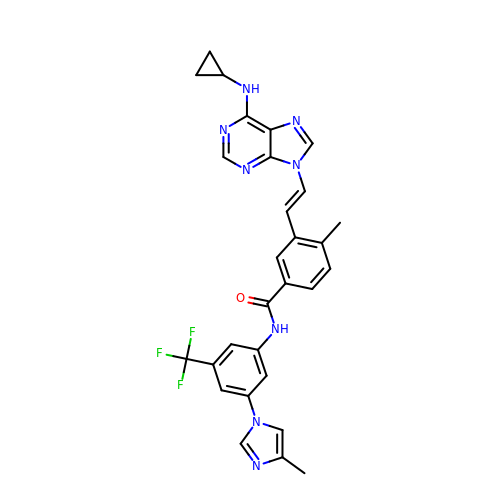3-{(E)-2-[6-(cyclopropylamino)-9H-purin-9-yl]ethenyl}-4-methyl-N-[3-(4-methyl-1H-imidazol-1-yl)-5-(trifluoromethyl)phenyl]benzamide | C29 H25 F3 N8 O | XQBYDVRVYRYLCH-BQYQJAHWSA-N>GINDLDISPIDPQTGGSFDQQGVFVKGYAMLGVTGQKGIDGSPDLDGQDE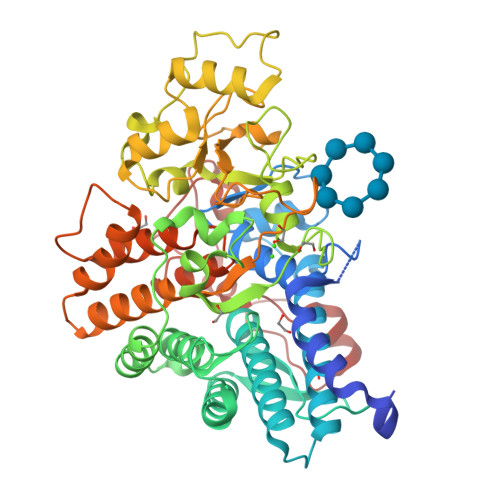GESGFYRTTFNCNELPTDECLWAWQKNQDIPQLTSISWSPSSQRTEWVYVRLGYDITQYNFFLDQTEGMTDAETLRQRAEIRFLRALHYWYFLDLFGKAPFKEHFSNDLPVEKKGTELYTYIQNELNEIEADMYEPRQAPFGRADKAANWLLRARLYLNAGVYTGQTDYAKAEEYASKVIGSAYKLCTNYSELFMADNDENENAMQEIILPIRQDGVKTRNYGGSTYLVCGTRVAGMPRMGTTNGWSCIFARAAMVQKFFSNLEDVPMLPADVEIPTKGLDTDEQIDAFDAEHGIRTEDMIKAAGDDRALLYSGVGGGRRKIQTDAISGFTDGLSIVKWQNYRSDGKPVSHATYPDTDIPLFRLAEAYLTRAEAIFRQGGDATGDINELRKRANCTRKVQTVTEQELIDEWAREFYLEGRRRSDLVRFGMFTTNKYLWDWKGGAMNGTSVASYYNKYPIPVSDINNNRNMSQNEGYK[2x]>[2x]MVREAGEVVAIVPAAGSGERLAVGVPKAFYQLDGQTLIERAVDGLLDSGVVDTVVVAVPADRTDEARQILGHRAMIVAGGSNRTDTVNLALTVLSGTAEPEFVLVHDAARALTPPA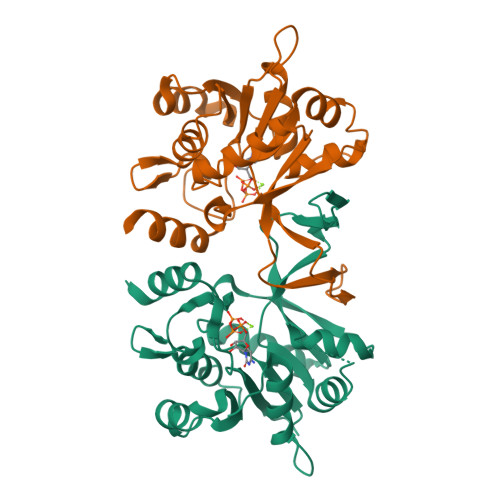LVARVVEALRDGYAAVVPVLPLSDTIKAVDANGVVLGTPERAGLRAVQTPQGFTTDLLLRSYQRGSLDLPAAEYTDDASLVEHIGGQVQVVDGDPLAFKITTKLDLLLAQAIVHHHH> MESXXXXXXXXXXXXXXXXXXXXXAKLLWLPLPMLMMLIVATVGVLVAVWLERKISAAVQQRIGPEYIGPLGILAPLADGLKLIFKEDVLPANSDRWLFTLGPAVVVIPVFLSYIIVPFGQNLLISNLAMGVFLWIALSSIAPIGLLMAGYASNNKYSLLGGLRAAAQSISYEIPLALAVLAVAMMSNGLGTVEIV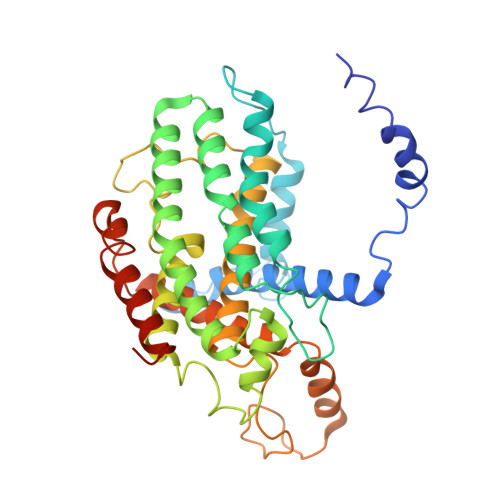EQQSQYGILSWNVWRQPIGFLVFWIAALAECERLPFDLPEAEEELVAGYQTEYAGMKFALFYLGAYVNLVLSALLVSVLYFGGWSFPIPLETIANLLGVSETNPFLQIAFAVLGITMTLIKAYFFVFLAILLRWTVPRVRIDQLLDLGWKFLLPVGLVNLLLTAGLKLAFPVAFGG>GGSHDCAKVDLENAELRRKLIRTKRAFEDTYEK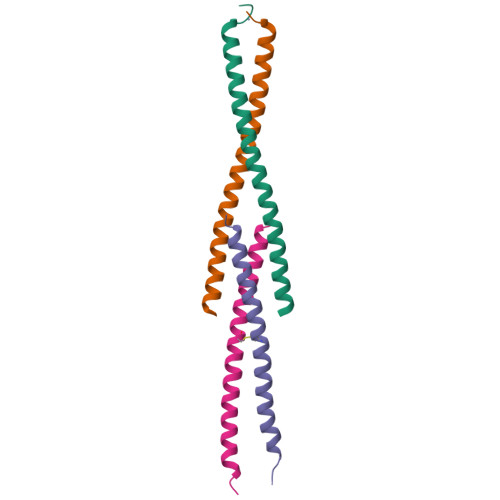LRMANKAKAQVEKDIKNQILKTHNVLRNVRSNMENEL[2x];>[2x]GPMDQQNSAVIGQLRLELQQARTEVETADKWRLECIDVCSVLTNRLEEEAGFLNSLLK The cou gene cluster includes couR, predicted to encode a MarR-family transcriptional regulator. The CouR regulon was defined by mapping CouR-binding sites to the cou promoters and demonstrating that CouR acts as a repressor. Consistent with the EMSA data, CouR did not detectably bind either p-coumarate or CoASH. Together, these data demonstrated that the effector of CouR is a p-hydroxycinnamoyl–CoA, the product of the CouL-catalyzed reaction. The CouR protomer showed the α1-α2-β1-α3-α4-β2-β3-α5-α6 secondary structure topology typical of MarR-family proteins.

To determine the molecular basis for recognition of p-coumaroyl–CoA by CouR and its potential effects on the conformation of this repressor, we determined a crystal structure of the CouR–p-coumaroyl–CoA complex to 1.52 Å resolution. The AU of the CouR–p-coumaroyl–CoA structure contained a single CouR dimer (Chains A and B) and two molecules of p-coumaroyl–CoA. The p-coumaroyl–CoA ligands bound in the central cavity formed between the two chains of the CouR dimer. The phenolic moiety of each of the ligands occupied equivalent hydrophobic pockets deep within each CouR protomer. Indeed, the phenolic hydroxyl formed hydrogen bonds with Asp10A and His117B of the different protomers. In contrast to the buried phenolic moieties, the CoA moieties of the ligands were solvent-exposed on the surface of the groove formed between the two wHTH motifs. Strikingly, the two CoA moieties adopted different configurations: one of the ligand molecules was bound in an ‘extended’ configuration along the α1 helix while the other adopted a ‘bent’ conformation with its adenyl group curved back and inserted between the pantothenyl regions of the two ligands. Despite these differences, the six phosphates of the two ligand molecules were nearly collinear, occupying the length of the groove formed between the two protomers of CouR, and were fully solvent exposed. Superposition of individual protomers of the CouR dimer (i.e., Chain A or Chain B) with a single protomer of ligand-bound CouR (Chain A) yielded RMSD values of 0.81 and 0.82 Å over 112 and 118 matching α-carbon atoms, respectively, indicating that at the level of a single chain, CouR does not undergo significant conformational change upon binding of p-coumaroyl–CoA. More significantly, the structural data combined with the functional characterization of the CouR variants strongly indicate that the anionic, bulky CoA moiety of p-hydroxycinnamoyl–CoA prevents the binding of DNA by steric occlusion and charge repulsion.

>MAESQALSDDIGFLLSRVGGMVLGAVNKALVPTGLRVRSYSVLVLACEQAEGVNQRGVAATMGLDPSQIVGLVDELEERGLVVRTLDPSDRRNKLIAATEEGRRLRDDAKARVDAAHGRYFEGIPDTVVNQMRDTLQSIAFPTFVE[2x]> RPSWSPTQASGQTVLPFTGIDFRLSPSGVAVDSAGNVYVTSEGMYGRVVKLATGSTGTTVLPFNGLYQPQGLAVDGAGTVYVTDFNNRVVTLAAGSNNQTVLPFDGLNYPEGLAVDTQGAVYVADRGNNRVVKLAAGSKTQTVLPFTGLNDPDGVAVDNSGNVYVTDTDNNRVVKLEAESNNQVVLPFTDITAPWGIAVDEAGTVYVTEHNTN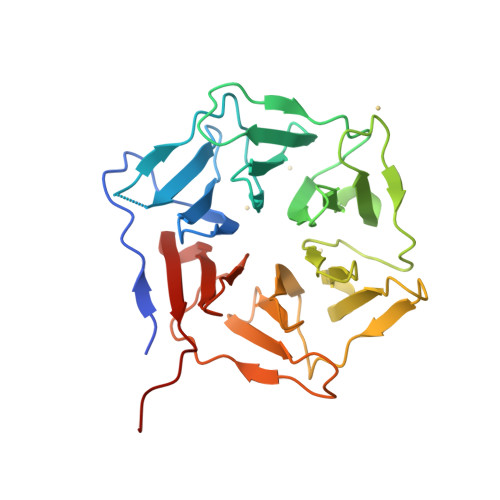QVVKLLAGSTTSTVLPFTGLNTPLAVAVDSDRTVYVADRGNDRVVKLTSLEHHHHHH>[2x]ISTLHHQTMPSDLTQDEFTQLSQSIAEFHTYQLGNGRCSSLLAQRI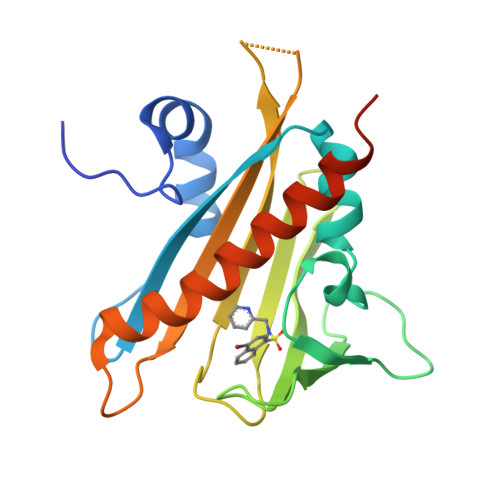HAPPETVWSVVRRFDRPQIYKHFIKSCNVSEDFEMRVGCTRDVNVISGLPANTSRERLDLLDDDRRVTGFSITGGEHRLRNYKSVTTVHRFEKEEEEERIWTVVLESYVVDVPEGNSEEDTRLFADTVIRLNLQKLASITEAMNRNNNNNNSSQVR>[2x]MEPTRIATNDRLSA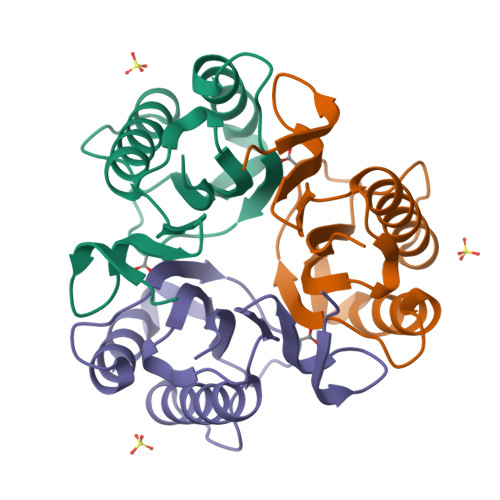AVCFDALVFLSGQVPGQAEDIHGQTREVLAKIDALLAEAGSRKERILSATIYLKDIARDFAALNEVWTQWLPTGQAPSRTTVQAELARPSVLVEITVVAARG4-chloranyl-2-cyclohexylsulfanyl-~{N}-(2-hydroxyethyl)-5-sulfamoyl-benzamide 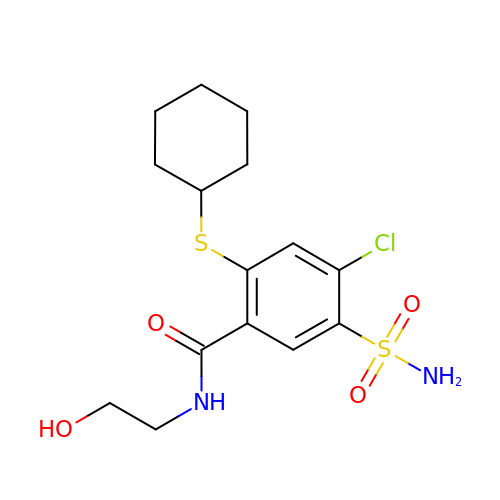| C15 H21 Cl N2 O4 S2 | PSEDAEWMXCWYRT-UHFFFAOYSA-N>[8x]MSDSQTLVVKLGTSVLTGGSRRLNRAHIVELVRQCAQLHAAGHRIVIVTSGAIAAGREHLGYPELPATIASKQLLAAVGQSRLIQLWEQLFSIYGIHVGQMLLTRADMEDRERFLNARDTLRALLDNNVVPVINENDAVATAEIKVGDNDNLSALAAILAGADKLLLLTDQKGLYTADPRSNPQAELI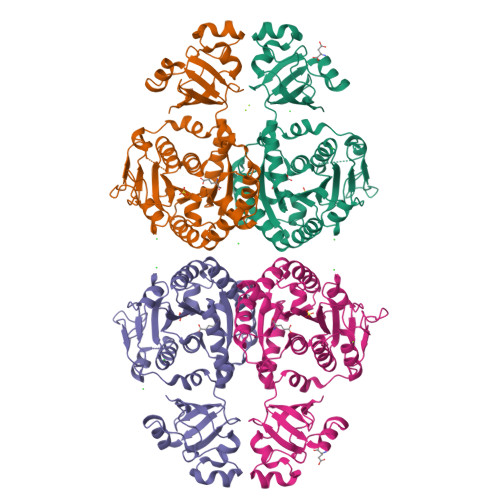KDVYGIDDALRAIAGDSVSGLGTGGMSTKLQAADVACRAGIDTIIAAGSKPGVIGDVMEGISVGTLFHAQATPLENRKRWIFGAPPAGEITVDEGATAAILERGSSLLPKGIKSVTGNFSRGEVIRICNLEGRDIAHGVSRYNSDALRRIAGHHSQEIDAILGYEYGPVAVHRDDMITR>[4x]PRHVRIKNWGSGMTFQDTLHHKAKGILTCRSKSCLGSIMTPKSLTRGPRDKPTPPDELLPQAIEFVNQYYGSFKEAKIEEHLARVEAVTKEIETTGTYQLTGDELIFATKQAWRNAPRCIGRIQWSNLQVFDARSCSTAREMFEHICRHVRYSTNNGNIRSAITVFPQRSDGKHDFRVWNAQLIRYAGYQMPDGSIRGDPANVEFTQLCIDLGWKPKYGRFDVVP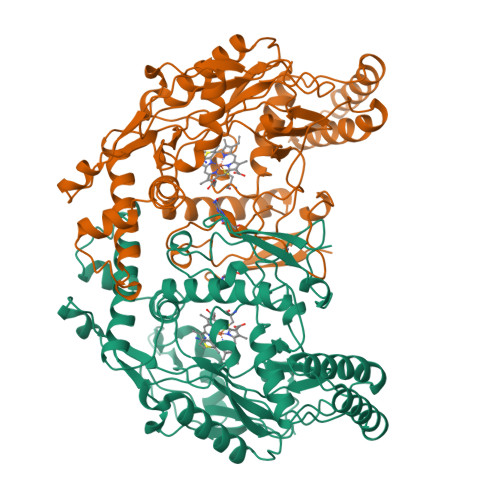LVLQANGRDPELFEIPPDLVLEVAMEHPKYEWFRELELKWYALPAVANMLLEVGGLEFPGCPFNGWYMGTEIGVRDFCDVQRYNILEEVGRRMGLETHKLASLWKDQAVVEINIAVIHSFQKQNVTIMDHHSAAESFMKYMQNEYRSRGGCPADWIWLVPPMSGSITPVFHQEMLNYVLSPFYYYQVEAWKTHVWQDEKRRP> MVTIVPYSHQYLKDICQLIQKDLSEPYSKYVYRYFVHQWPEFSFVALDNDRFIGAVICK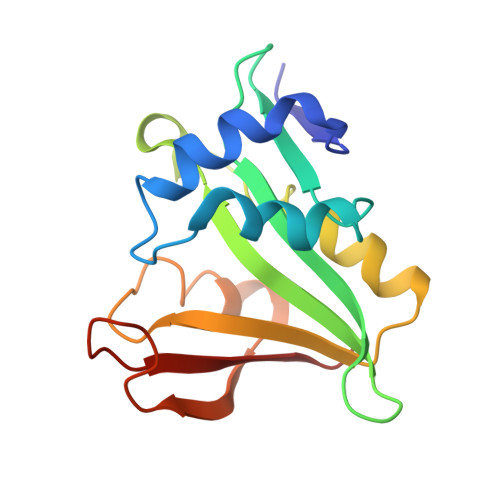QDVHRGTTLRGYIAMLAIVKEYRGQGIATKLTQASLDVMKNRGAQEIVLETEVDNEAAMSFYERLGFCRYKRLYRYYLNGTDAFRYILYPN>[2x]MSEECIENPERIKIGTDLINIRNKMNLKELIHPNEDENSTLLILNQKIDIPRPLFYKIWKLHDLKVCADGAANRLYDYLDDDETLRIKYLPNYIIGDLDSLSEKVYKYYRKNKVTIIKQTTQYSTDFTKCVNLISLHFNSPEFRSLISNK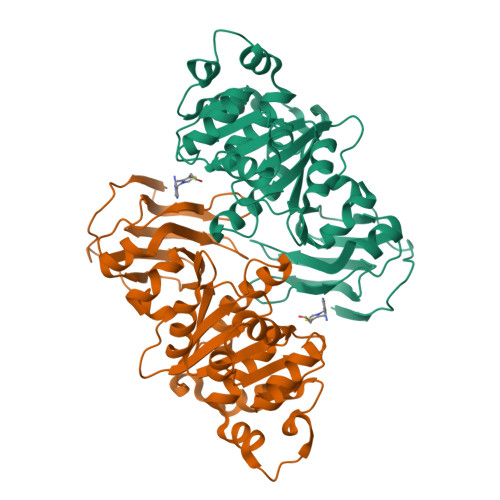DNLQSNHGIELEKGIHTLYNTMTESLVFSKVTPISLLALGGIGGRFDQTVHSITQLYTLSENASYFKLCYMTPTDLIFLIKKNGTLIEYDPQFRNTCIGNCGLLPIGEATLVKETRGLKWDVKNWPTSVVTGRVSSSNRFVGDNCCFIDTKDDIILNVEIFVDKLIDFL>[2x]MASDVNDNRPVFVRPPNGTILHIKEEIPLRSNVYEVYATDNDEGLNGAVRYSFLKTTGNRDWEYFTIDPISGLIQTAQRLDREKQAVYSLILVASDLGQPVPYETMQPLQVALEDIDDNEPLFVRPPKGSPQYQLLTVPEHSPRGTLVGNVTGAVDADEGPNAIVYYFIAAGDEDKNFHLQPDGRLLVLRDLDRETEATFSFIVKASSNRSWTPPRGPSPALDLLTDLTL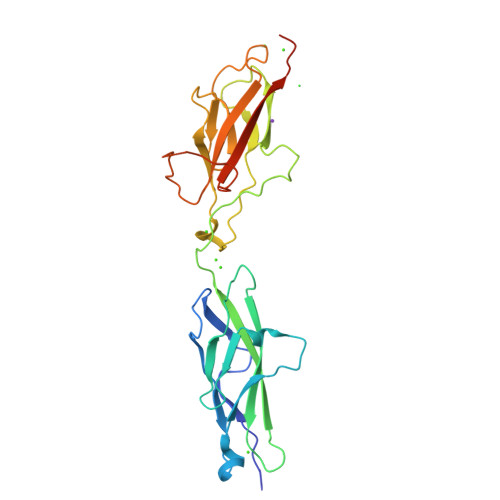QEVRVVLEDINDQLEHHHHHH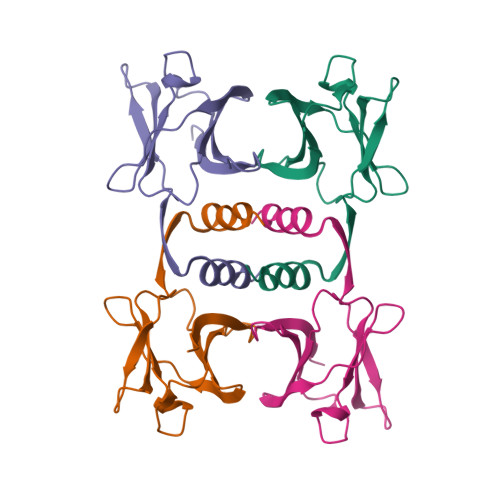>[4x]MATTNDSAVLFYIVASQKKLSFDYTPNWGRGSPNSYIDNLTFPRVLTNKPYKYRVVKAGQDLGVRDSYSVQSDGSQKVNFLEYNAGRGIADTQTIQVYVVDPDNGNQYLVAQWKLEHHHHHH>TAPKVLFTGVVDARGERAVLALGGSLAGSAAEASHLVTDRIRRTVKFLCALGRGIPILSLDWLHQSRKAGFFLPPDEYVVTDPEQEKNFGFSLQDALSRARERRLLEGYEIYVTPGVQPPPPQMGEIISCCGGTYLPSM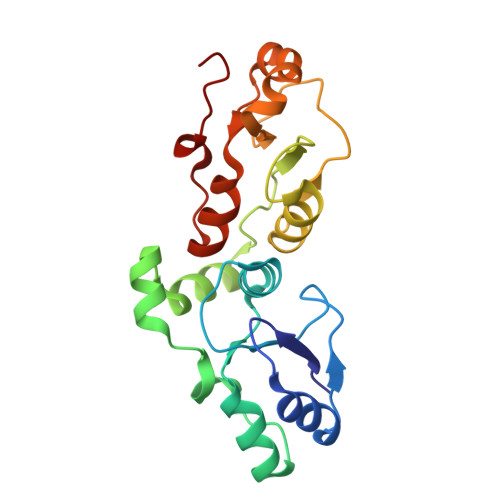PRSYKPQRVVITCPQDFPHCSIPLRVGLPLLSPEFLLTGVLKQEAKPEAFVLSPLEM[2x]>MATPVTIYGPPLCTAVSRVLATLIEKDVPFHLIPIDLSKGEQKKPEYLKIQPFGQVPAFKDESITLFESRAICRYICDKYADKGNKSLYGTDILSKANIDQWVETDGQTFGPPSGDLVHDLLFSSVPVDEALIKKNVDKLAKVLDIYEQKLGQTRFLAGDEFSFADLSHLPNGDYLVNSTDKGYLFTSRKNVNRWWTEISNRESWKKVLEMRKN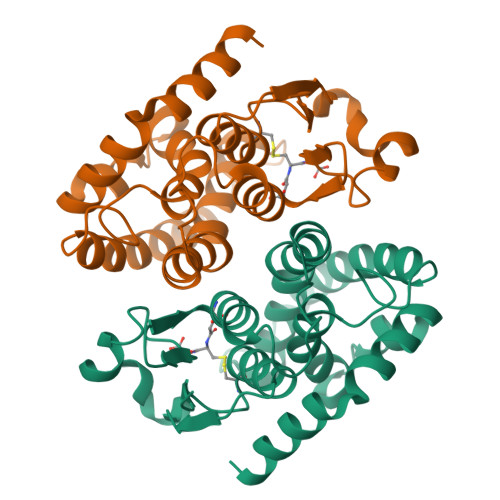A[2x]>[60x]MYFFSVDPRNGASKSGDVCGSCCCESISARPGEVNGVMVSYAAWSAPLRGHGLTNKTTFEIDGVSVTPPKVSNAFGRTKVGVVFEGTLSDLFPNPEGEQVEYEISELNGPSNGVVELGANGAFTYTPGALFTGVDRFWFSINGNIGEYVISVDPTTSELPQPPFTTPVYVPAARRSVDPRTHVLKFVLGVSPAAIPGDVYRLTVRQVAIDCDGNEFVHISCYDISIGSCG;>MLGIPLLTRKAALTPPAPSANPAKIFIRRFFSAGVAKNVVSYSNVMAAQRAMEHPVAFRCLDKLGLTVQSVKWDVGKDPQNTQVGDGGMSASQRKALQQILQRPNPTMSGAQLRYSAALSWACFGRMAFKVSVMSDGSVNAIWPLGIPFLKQKFDRYGDVESFQYGDEAGKETIPSFTKVEKNDKGRPIKNYAFMIVKPSINGAMNFDVQNTPLQAIGVPVALYDALMARAIDSADGTPNSKWLVTASRDLDDGQAKEVKEGIEETKPGGDNGGEIIFIAGTDVKVQEMKNDLSDIHSKVPLDDQARTIAGNFGIPIALLGFAGADGSKFANNYDESRKAFFEDTIEPGYLTPLEDGFSMFLCGAGYRVIFDRDSIPALRKSRADIAATYDKVTFITEEEKREVTGWPAKKEGQTQNDDA[12x];>MRTADRKHRVIVCSQQSDVDDEGRLLITRAGVIQGWAAIAPVKAIRFSQDGVSMQKDTMQPTHDITMNYNPDVNVSVSAWVYEHRLKSPPRWFKVLSVVNVDECSRYMKIRCRLVETSDDVTPPVEEEKNSFGAVKIDIPL[6x];>METKLTYGNRVTLPEFAKYIVAPAFHEIEGRAIPVTGVDDDASGTQATKLPFVLVGLRQGDTSGPATIAGNSTINLRDDFIVEFNMKKERYRDRKGGETPFFSYYDYESIRDRLFNSMIEFSGEHGITFEFVSLDISTEGDVVYIEFRFRQNYEWCETVREADTTIEAGRFSINLQGC[6x];>MACNKQNGVKNILITFTDCDTQEVIGPISHEQPDDTLPTYKNCAWTNTALTNGYVQRSASNATMTLPVVRDLRVPLAFYQGCAQVDVQVEKFDGTVMTLTEGAVVEPEESDGRSVTMNIVASEIDELLPPGSLAAA[6x];>MNLDTLLPLQTIREHAKCDDNPRVTDDLLKLYREAAFEAAELYTGLSFTPEKTIVEPIRLKGRRGKIILSATPIAGRPVVFYGGGLGSPLELIPRPGSNVLFFPYGSPDRFQTWGDCHTCDVESQLMATYVTGRRCENSVPAGIIIGILKLIAWNINNPGDEVMSVRNTLNANAQGLIGGTNNGAVISGAQDEWFRYRRVLL[12x];>[25x]MVKLNCRPLCQAPTASRLVSPPCFICRGVAPSAPVTPG;>MDCRNLCGAAAPSRLVQPGCFICRGVAVSIPPAAPGPATSVFDTPPSTFSLRPDGTIIAGTGIRGDHASVGTDGTIEMFIVPFIGDVTGSELTHPYAVELQDGEELAIAFGVTLKSGYGARITEYYDVSLFLENGGNSKELTLQPANTKSGYVWSDGHGYNITDSDGDLHTVQNVTRPVWFEMTEPGIVGVIMEARYKATGLVSSSISITVNVTYAD[5x];>MANKESELNGLDDIHSDIEKLSAHVEKFSDGMDEKYKELTARFDGVKGDNDAIRKAVADATKEYAELSAKHQFFTEELAAMKARLDTPIMRSQAELDDHDRKTAIQLQRNMHEFRGGDPKEFVADESNLVDLKAYRSAVRKMLKVGIESKERVIASMTDVERKAFEASTIGPAFFTPQVLALEVDCNIECASLLDLYGQIEVSRSTFTYMKIADYGQLGEYTCDAKCDAEFGEPGNIRHLEGKTYDYRGVFCFNRKNLQEANYDFLSFMIGAAQRSHRINRNQALMIGKGVNEPKGWLTENCFPVFQTLPVDVNGTSTPAFLAQDWRRFVTSFPAEYGEARSVMHQNVFGYLAAMVDANGRFLFGDGDLTFTPDLVRERIRISNCLPDPTEGNTKGGTGQDAFAAGSFVAAQAAWKTAFYAVEKRPMFFEQYEGGSSAWCVKYQFGAEDGGFVGCCEHGRILQIG[30x];>[40x]MNFNVGVDFPSFIAWDGEESFPVKVDGFNQFGFTFKTIAALTAATTFNIFYHEPSDADPCVPGPAIRVPEVPFCDTVLLSEDGLAAVTLPETVTPDSFCAGTVPCMNGQWISIAPATGSETNAANVQITVTMKGATR

Caudovirales, the taxonomic order for the tailed double-stranded DNA bacteriophages, is characterized by the presence of a tail—a host cell attachment organelle that is connected to the genome-containing spherical or elongated capsid via a neck. We describe cryo-EM structures of the neck, the neck-capsid and neck-tail junctions, and capsid of the Agrobacterium phage Milano. The tail to capsid junction involves a symmetry mismatch that is bridged by the neck, and is therefore crucial for the assembly of tailed phage. The extensive network of disulfide bonds within and between neck, collar, capsid and tail provides an exceptional structural stability to Milano.

A 3-fold symmetrized map focused at the neck-tail junction was used to understand the interactions between the collar and the tail. Finally, a no-symmetry-imposed map was used to generate an atomic model of the complete neck. We describe how the neck 1 protomers undergo structural polymorphism to connect the 12-fold neck with the 5-fold capsid vertex. The 12 ring-forming gp14 protomers exhibit structural polymorphism. Their β-sandwich domains adopt different orientations in each protomer and can be described as 12 steps in a continuous tilting relative to the α-helical domain. When the α-helical domains of the 12 gp14 subunits are superimposed, they display an RMSD of 2.6 Å, while the β-sandwich domains have a varying orientation with the maximal distance between their distal parts reaching 24 Å. The β-sandwich domains are clustered in three groups with 3, 4, and 5 members each creating a 12-to-5-fold symmetry adaptor assembly to bridge neck-capsid symmetry mismatch. Five out of 12 gp14 β-sandwich domains (n, n + 2, n + 5, n + 7, n + 10, CCW direction looking from the capsid side) display pseudo-5-fold symmetry. These domains are covalently linked to the MCP (gp9) by two disulfide bonds, gp14Cys117– gp9Cys252 and gp14Cys120– gp9Cys440, which emanate from a head joining loop of the β-sandwich domains. The head joining loops of the remaining seven gp14 protomers are not resolved in our maps and thus likely to be disordered. In summary, in the gp14 neck 1 dodecamer, the α-helical domain connects the portal to neck 1 ring smoothly while maintaining C12 symmetry, while its β-sandwich domain binds to the five-fold symmetric capsid vertex by adopting 12 different conformations.Purine nucleoside phosphorylases (PNPs, EC 2.4.2.1) are cytosolic enzymes involved in the purine salvage pathway metabolism in most organisms. The enzyme degrades (2′-deoxy)nucleosides based on 6-oxopurines to the corresponding purine bases and (2-deoxy)ribose-1-phosphate. Purine nucleoside phosphorylase (PNP) is a well-known molecular target with potential therapeutic applications in the treatment of T-cell malignancies and/or bacterial/parasitic infections. The results are supported by a crystallographic study of eight enzyme-inhibitor complexes and by ADMET profiling in vitro and in vivo.

To obtain information on the binding pose and interacting residues, crystal structures of recombinant hPNP in complex with inhibitors 18c, 45b, 45q, 45i, and 45n were determined and refined to high resolution. All five inhibitors bind to hPNP in a similar way, i.e., through seven direct hydrogen bonds and four water-mediated hydrogen bonds as well as numerous hydrophobic interactions. The methoxy group at position C5 of phenyl moiety of 45b interacts with both Phe200 and Phe159 from molecule B. Bromide substitution at position C4 in 45q interacts with His257, Val260, and Leu261 of the helix (residues 257–267 are disordered in apoenzyme and form a helical structure, which elongates C-terminal helix upon substrate/inhibitor binding so this region will be referred to as helix), while central phenyl moiety interacts with Val260. Bromide substitution at position C4 of 45q leads to a 2–3-fold decrease in affinity toward hPNP. The presence of a bromide substituent that interacts with helix causes a shift in the position of the central phenyl moiety and the substituent points toward helix. No halogen bond interaction of bromine was detected in the crystal structure; the substitution pose however forces rearrangement of the His257 sidechain, whose position is disordered and cannot be unambiguously modeled based on the electron density map. Similar outcomes were observed for bromo-derivatives 45p–q , which exhibited similar cellular activity, with compound 45q being the most active from the series (CCRF-CEM IC50 = 9 nM).

> MENGYTYEDYKNTAEWLLSHTKHRPQVAIICGSGLGGLTDKLTQAQIFDYGEIPNFPRSTVPGHAGRLVFGFLNGRACVMMQGRFHMYEGYPLWKVTFPVRVFHLLGVDTLVVTNAAGGLNPKFEVGDIMLIRDHINLPGFSGQNPLRGPNDERFGDRFPAMSDAYDRTMRQRALSTWKQMGEQRELQEGTYVMVAGPSFETVAECRVLQKLGADAVGMSTVPEVIVARHCGLRVFGFSLITNKVIMDYESLEKANHEEVLAAGKQAAQKLEQFVSILMASIPLPDKAS>[4x]SHMKIGVF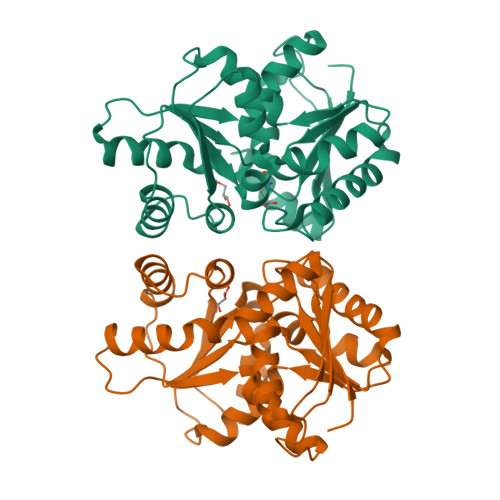DSGVGGFSVLKSLLKAQIFDKIIYYGDSARVPYGTKDPTTIKQFGLEALDFFKPHKIELLIVACNTASALALEEMQKHSKIPIVGVIEPSILAIKQQVKDKNAPILVLGTKATIQSNAYDNALKQQGYLNVSHLATSLFVPLIEENILEGELLETCMRYYFTPLEILPEVVILGCTHFPLIAQKIEGYFMEHFALSTPPLLIHSGDAIVEYLQQKYTLKKNACTFPKVEFHASGDVVWLEKQAKEWLKL>GPLGSPEFPGEFYIPPEPSNDAIEIFSSGIASGIHFSKYNNIPVKVTGSDVPQPIQHFTSADLRDIIIDNVNKSGYKIPTPIQKCSIPVISSGRDLMACAQTGSGKTAAFLLPILSKLLEDPHELELGRPQVVIVSPTRELAIQIFNEARKFAFESYLKIGIVYGGTSFRHQNECITRGCHVVIATPGRLLDFVDRTFITFEDTRFVVLDEADRMLDMGFSEDMRRIMTHVTMRPEHQTLMFSATFPEEIQRMAGEFLKNYVFVAIGIVGGACSDVKQTIYEVNKYAKRSKLIEILSEQADGTIVFVETKRGADFLASFLSEKEFPTTSIHGDRLQSQREQALRDFKNGSMKVLIA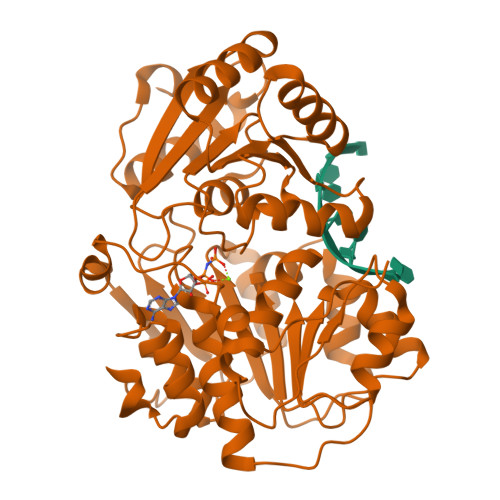TSVASRGLDIKNIKHVINYDMPSKIDDYVHRIGRTGRVGNNGRATSFFDPEKDRAIAADLVKILEGSGQTVPDFLRTC[4x]>[6x]SLSTIICIGMAGSGKTTFMQRLNSHLRAEKTPPYVINLDPAVLRVPYGANIDIRDSIKYKKVMENYQLGPNGAIVTSLNLFSTKIDQVIRLVEQKKDKFQNCIIDTPGQIECFVWSASGAIITESFASSFPTVIAYIVDTPRNSSPTTFMSNMLYACSILYKTKLPMIVVFNKTDVCKADFAKEWMTDFESFQAAIKEDQDGYMSSLVNSMSLMLEEFYSQLDVVGVSSF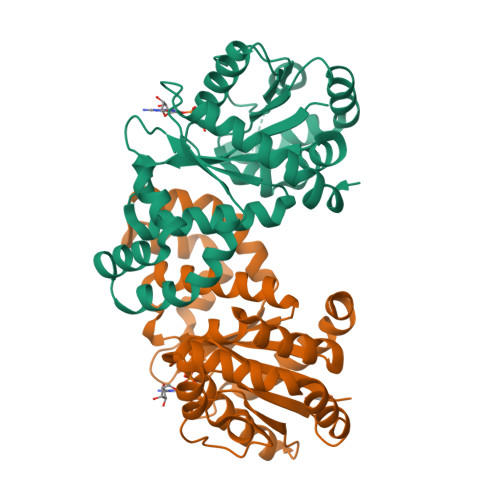TGDGFDEFMQCVDKKVDEYDQYYKKHHHHHH> MNVNNPNQMTVTPVYNGCDSGEGPQSVRGYFDAVAGENVKYDLTYLADTQGFTGVQCIYIDNAENDGAFEIDVEETGQRIKCPAGKQGYFPLLVPGRA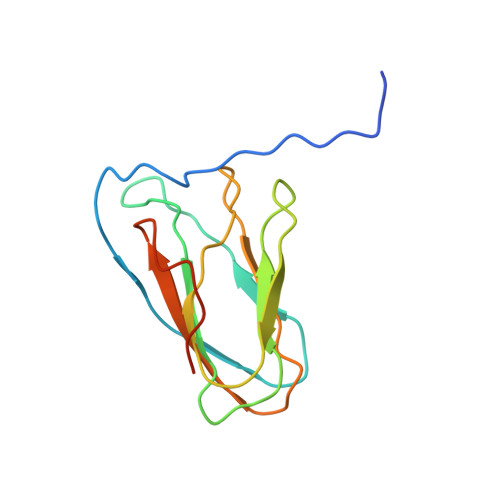KFVARHLGSGKKSVPLFFLNFTIAQGVW>FDRDRLFSVVSRGVPEELTGLLEYLRWNSKYLTDSAYTEGSTGKTCLMKAVLNLQDGVNACIMPLLQIDKDSGNPKPLVNAQCTDEFYQGHSALHIAIEKRSLQCVKLLVENGADVHLRACGRFFQKHQGTCFYFGELPLSLAACTKQWDVVTYLLENPHQ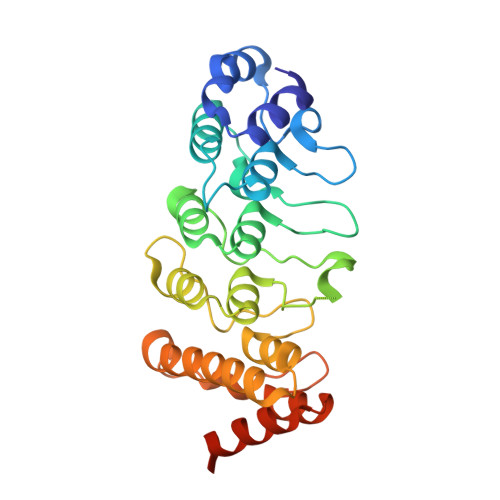PASLEATDSLGNTVLHALVMIADNSPENSALVIHMYDGLLQMGARLCPTVQLEEISNHQGLTPLKLAAKEGKIEIFRHILQREFSGAAAHHHHHH[2x]> 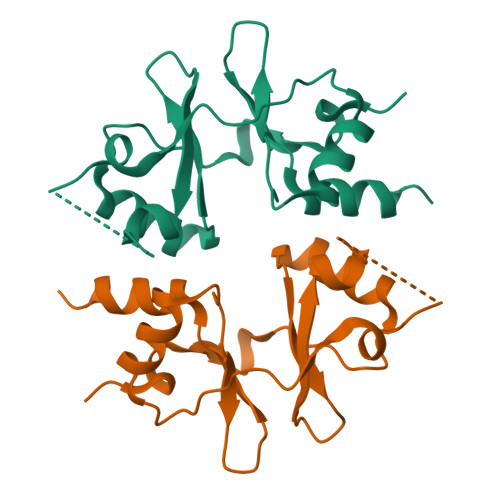GSGVYTVGEFMTKKEDLHVVKPTTTVDEALELLVENRITGFPVIDEDWKLVGLVSDYDLLALDSISGSGRTENSMFPEVDSTWKTFNAVQKLLSKTNGKLVGDLMTPAPLVVEEKTNLEDAAKILLETKYRRLPVVDSDGKLVGIITRGNVVRAALQIKRSGDRNA> GAMSNQHVLEEKTVAGWVAENQTA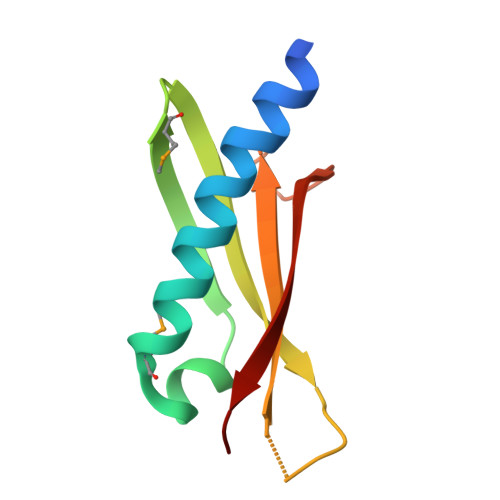LLYLMTRGQRAVRQQGESDMAGSRWYWRTTPLSTGNALLQAVDIEVSLHEDFSSVIQSRRAWFSA(2S)-2-phenyl-N-[(1R)-1-phenylethyl]propanamide | C17 H19 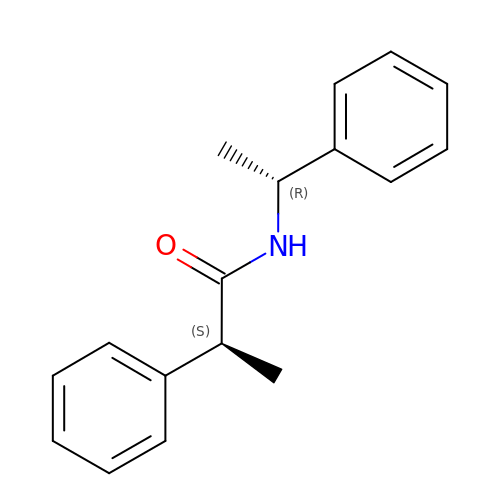N O | ZWNCJNODOVPNTF-UONOGXRCSA-N>LRSRRVDVMDVMNRLILAMDLMNRDDALRVTGEVREYIDTVKIGYPLVLSEGMDIIAEFRKRFGCRIIADFKVADIPETNEKICRATFKAGADAIIVHGFPGADSVRACLNVAEEMGREVFLLTEMSHPGAEMFIQGAADEIARMGVDLGVKNYVGPSTRPERLSRLREIIGQDSFLISPGVGAQGGDPGETLRFADAIIVGRSIYLADNPAAAAAGIIE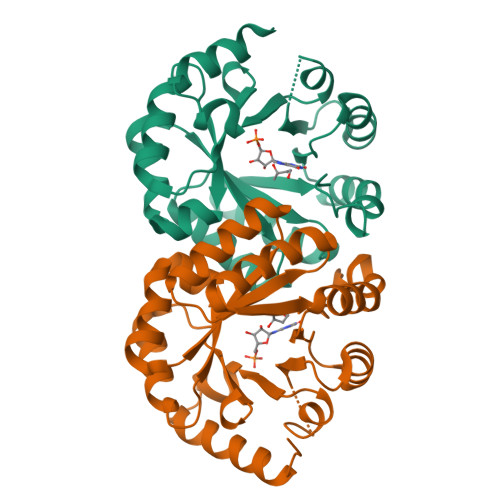SIKDLLIPE[2x]>MSRLYKDICSLRTLYGAWRKVRSSAFLSSSDEIRREAEEFESRLPDSLIEIQHALSKQIFIFLQQTGVAQKKPGGKSRPLVLAPIPNRVVQRALLDVLQRRVRLVKRVLGTPTSYGGIPDKRVAMAIADAREAMRTGARFHIRSDIPAFFTKINKDRVLELLRPHLNCEATLKLFEEAIRTDLANIDDLRRKGLDEIFPIGIEGVAQGSPLSPLLANIYLADFDLAMNSNGITCLRYIDDFLLLGASLSDVDKAFNRALKELGKIGLEAYDPRTDKTKASRGATEIGFDFLGCNVSPGLIQPSEATRRRFRAKLDAEFVAASHALRYNAQYQDGDGKYSYSSALYRIDKIILGWGKAFTFCNGSQCMIALDDFISNKLAQLEAEKIAILANSDSTVRRRVLGVRLLIDIQN[2x]

Bacteria encode a variety of reverse transcriptases (RTs) that evolved from mobile group II intron RTs to perform different cellular functions. In a previous study, we showed via genetic and biochemical analyses that a Pseudomonas aeruginosa group II intron–like (G2L4) RT functions in DSBR via MMEJ both in its native host and when transferred into Escherichia coli. Here, we determined a 2.6-Å crystal structure of a full-length G2L4 RT apoenzyme and a 2.8-Å cocrystal structure of G2L4 RT bound in an active conformation to a snapback DNA synthesis substrate and incoming dNTP. All RTs share a common structural framework composed of fingers, palm, and thumb or thumb surrogate regions that fold into a hand-like structure, forming a cleft containing an RT active site composed of three conserved aspartate residues that bind catalytic Mg2+ ions.

The structure was solved at 2.60-Å resolution in space group P21 by de novo phasing using selenomethionine. Unlike group II intron RTs, which typically appear in crystal or cryo-EM structures as monomers, the G2L4 RT apoenzyme structure revealed two monomers per asymmetric unit forming a symmetric dimer, a difference verified by size-exclusion chromatography comparing G2L4 RT to a closely related mobile group II intron RT (Geobacillus stearothermophilus group IIC intron RT, denoted GII RT). Continuous density could be traced for all amino acids, except those in two putative loops (Q65 to R78 in RT1 and G116 to D120 in RT2a). The two G2L4 RT monomers that form the apoenzyme dimer have nearly identical hand-like folds composed of fingers, palm, and thumb regions (RMSD = 0.83 Å for main chain carbon atoms), but lack DNA-binding (D) or DNA endonuclease (En) domains found in group II intron RTs. The thumb domain of G2L4 RT is similar to that of GII RT in being composed of three parallel α-helices (α1-3), but differs in extending straight up for 41 Å, 15 Å farther than in GII RT, and ending with additional short α-helices (α4 and α5) that interact with the thumb domain of the opposite monomer. RT2a is nearly identical to that in the GII RT cocrystal structure, but with a hinge region (G116 to D120) that connects to RT2 and is disordered in the absence of bound substrate. By contrast, RT3a in G2L4 RT differs markedly from that in group II intron RTs in forming a novel structural feature, a double-helical plug (denoted RT3a plug; highlighted in purple in Fig. 1 C and E). The RT3a plug is a structural adaptation that completely blocks the active site of G2L4 RT, rendering the apoenzyme inactive until it encounters a physiological substrate, as described further below. The structure of the RT3a plug and its binding in the active-site pocket of G2L4 RT are stabilized by an interaction network that includes salt bridges formed by two conserved arginine residues (R190 and R191) that are located within the 9-aa insertion and form part of the first α-helix of the RT3a plug.> MQKTLEVWIMPNSPQPAEDFKALVAPFEKAHGVEVKVTVLDAGVAWTKITTAATSGVGPDLTQLGTTWVGAISAMGVLEPVDDVLEALGGEKAYLPAVWRTTRLEGARQATAVPWFSELRAFYYRTDALKAAGVNPAEMFASWQGFEAGLARLKASSFRDPETKAPLAPLCTPGKNSWDVLHNAAPWIWGAGGEIVRQAGGRWQSALNSPESLEGLYFFLSLAQKGYVPAESLEKNTAQIEADFQAGKCAVFASGPWMIQRAQVPEAKGGFAERTAAKNLGVAPYPAGPKGRYTFFGGSNLALFNFSKNKPLAKELLKYLGGPEAQVRYAQMTGMLPALRSAWSDPSFQQNPLLRTFIQAAQFGRTYPSLAGWGGVENLAV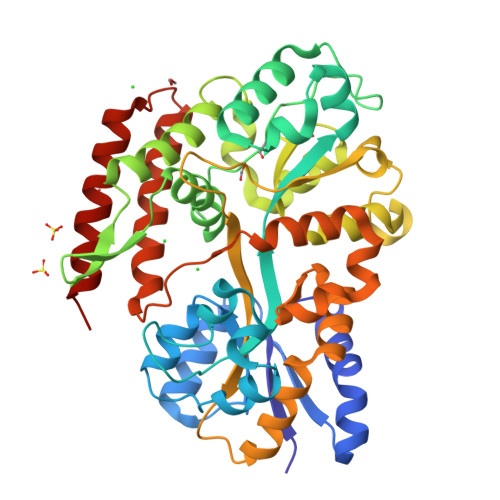QHLGMAWDLVAQGRLTREALKDLMDKASAAINQALRHHHHHH> GPTIYHAKDAVQTTKPSERKPRLVVFVVGETARADHVQFNGYGRETFPQLAKVDGLANFSQVTSCGTSTAYSVPCMFSYLGQDDYDVDTAKYQENVLDTLDRLGVGILWRDNNSDSKGVMDKLPATQYFDYKSATNNTICNTNPYNECRDVGMLVGLDDYVSANNGKDMLIMLHQMGNHGPAYFKRYDEQFAKFTPVCEGNELAKCEHQSLINAYDNALLATDDFIAKSIDWLKTHEANYDVAMLYVSDHGESLGENGVYLHGMPNAFAPKEQRAVPAFFWSNNTTFKPTASDTVLTHDAITPTLLKLFDVTAGKVKDRAAFIQ

A key colistin resistance mechanism is the production of MCR-1, a plasmid-encoded phosphoethanolamine transferase that has disseminated worldwide. MCR-1 catalyses the transfer of positively charged phosphoethanolamine onto lipid A, which is subsequently incorporated into the outer membrane, reducing the net negative charge and preventing colistin binding. It is an integral, metal-dependent inner-membrane protein, with a large periplasmic domain containing the catalytic centre and the conserved Thr285 that is likely to act as the acceptor for the phosphoethanolamine group during the transfer reaction.

To understand MCR diversity, we have solved the crystal structure of the MCR-2 catalytic domain (residues 217–538; MCR-2CD), which is 87% identical to MCR-1CD. As for Zn1 in MCR-1, Zn1 in MCR-2 is coordinated by Glu246, Thr285 and Asp465 (all with a coordination distance of 1.92 Å) and His466 (2.04 Å) in a tetrahedral geometry. Although the Zn1 coordination distances are shorter in MCR-2 compared with MCR-1 (Hinchliffe et al., 2017), there are no other structural differences around the Zn1 site, further underlying the importance of Zn1 to enzyme function. Solvent-accessible loops are largely unperturbed, although loop 411–424 shifts ∼4 Å between MCR-15GRR and MCR-2CD. A single residue (Ser330) is a Ramachandran plot outlier, with φ and ψ values of −165.9 and −82.4°, respectively. This residue is sterically strained by forming a hydrogen bond to Asn329, and is also a Ramachadran plot outlier in all other MCR-1 structures. The MCR-2CD structure also indicates that amino-acid mutations on the periplasmic facing surface of MCR-1 are well tolerated. The physiological relevance of the second zinc site has yet to be established, although it has now been observed in three MCR crystal structures. Resolving this issue will require accurate and detailed mechanistic and computational studies of phosphoethanolamine transfer by the MCR family of enzymes, the latter of which will be greatly facilitated by the exceptionally high resolution of the current structure.>MGSSHHHHHHSSGLVPRGSHMFHYHERELESEEGFM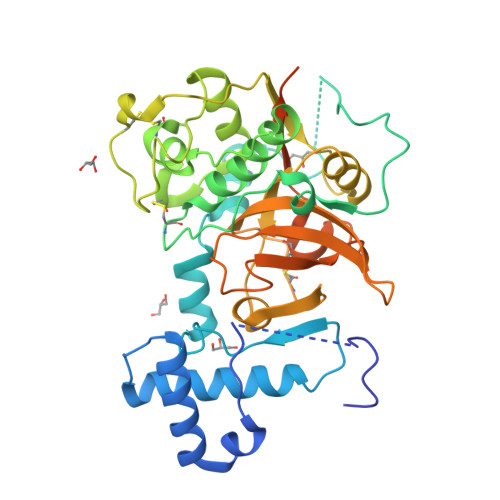GMYDRWREQHNIEMRSPERFNVFKYNVRRIHESNKMDKPYKLKVNEFADMTNLEFVNTYANSKISHFQALRGSAPGSIDTDPNKDFIYANVTKIPDKVDWREKNAVTDVKGQGGCGSCWAFAAVVALEGINAIRTGKLVKFSEQQLVDCDMTNAGCDGGLMEPAFTYVIKHGGIAPEASYPYVGKRETCDKAKIKDVLKIDGRQNVPGLDEEALRKAVAHQPVATGIQLSGHGLQFYSEGVYTGDCGTEPNHGVGIVGYGENEKGIKFWTVKNSWGPTWGEKGYIHLQRGARKEGLCGVAMHSSFPIMNDPNPPKDDPNGPKDDPDAPKDPKFKTTQRLQGIRTKLLEL[2x]> MSEAEARPTNFIRQIIDEDLASGKHTTVHTRFPPEPNGYLHIGHAKSICLNFGIAQDYKGQCNLRFDDTNPVKEDIEYVESIKNDVEWLGFHWSGNVRYSSDYFDQLHAYAIELINKGLAYVDELTPEQIREYRGTLTQPGKNSPYRDRSVEENLALFEKMRAGGFEEGKACLRAKIDMASPFIVMRDPVLYRIKFAEHHQTGNKWCIYPMYDFTHCISDALEGITHSLCTLEFQDNRRLYDWV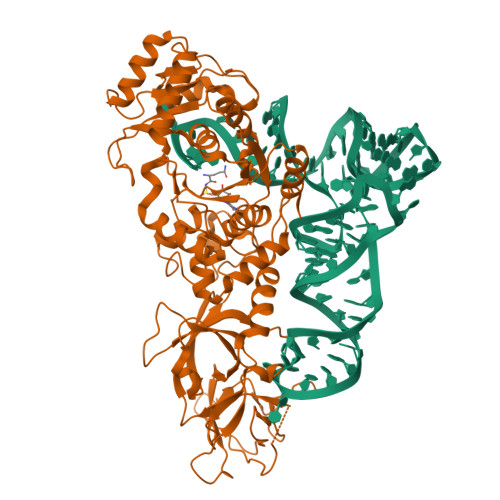LDNITIPVHPRQYEFSRLNLEYTVMSKRKLNLLVTDKHVEGWDDPRMPTISGLRRRGYTAASIREFCKRIGVTKQDNTIEMASLESCIREDLNENAPRAMAVIDPVKLVIENYQGEGEMVTMPNHPNKPEMGSRQVPFSGEIWIDRADFREEANKQYKRLVLGKEVRLRNAYVIKAERVEKDAEGNITTIFCTYDADTLSKDPADGRKVKGVIHWVSAAHALPVEIRLYDRLFSVPNPGAADDFLSVINPESLVIKQGFAEPSLKDAVAGKAFQFEREGYFCLDSRHSTAEKPVFNRTVGLRDT>MTVQAQNIDAITAGAMPHEEPELTDGFHLVIDALKLNGIETIYNVPGIPITDLGRLAQAEGLRVISFRHEQNAGNAAAIAGFLTKKPGICLTVSAPGFLNGLTALANATTNCFPMILISGSSEREIVDLQQGDYGEMDQLAIAKPLCKAAFRVLHAADIGIGVARAIRAAVSGRPGGVYLDLPAKLFSQVIDADLGAR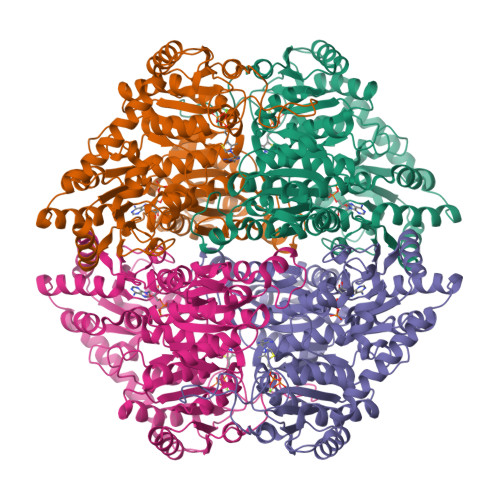SLVKVIDAAPAQLPAPAAIARALDVLKSAERPLIILGKGAAYAQADEAVRALVEESGIPYVPMSMAKGLLPDTHPLSAGAARSTALKDSDVVLLVGARLNWLLSHGKGKTWGEPGSKRFIQIDIEPREMDSNVEIVAPVVGDIGSCVEALLDGIRKDWKGAPSNWLETLRGKREANIAKMAPKLMKNSSPMCFHSALGALRTVIKERPDAILVNEGCNTLDLARGIIDMYQPRKRLDVGTWGVMGIGMGFAVAAAVETGKPVLAVEGDSAFGFSGMEVETICRYELPVCIVIFNNNGIFRGTDTDPTGRDPGTTVFVKNSRYDKMMEAFGGVGVNVTTPDELKRAVDEAMNSGKPTLINAEIDPAAGSEGGNIGSLNPQSTLKKK[8x]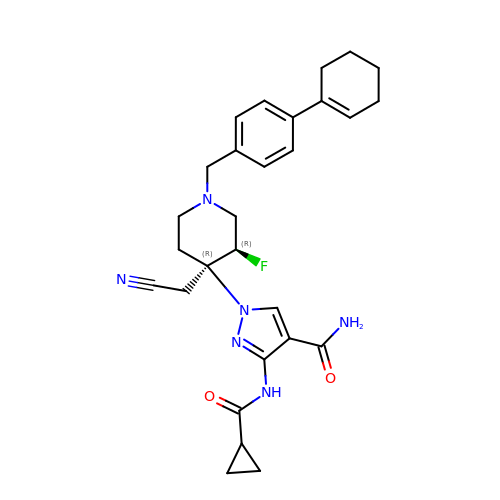1-[(3~{R},4~{R})-4-(cyanomethyl)-1-[[4-(cyclohexen-1-yl)phenyl]methyl]-3-fluoranyl-piperidin-4-yl]-3-(cyclopropylcarbonylamino)pyrazole-4-carboxamide | C28 H33 F N6 O2 | JZLQNFWWJFOUEZ-YWEHKCAJSA-N>[2x]SNAMLDITTITRQNVTSVVGYYSDAKDDYYSKDSSFTSWQGTGAEALGLSGDVESARFKELLVGEIDTFTHMQRHVGDAKKERLGYDLTFSAPKGVSMQALIHGDKTIIEAHEKAVAAAVREAEKLAQARTTRQGKSVTQNTNNLVVATFRHETSRALDPDLHTHAFVMNM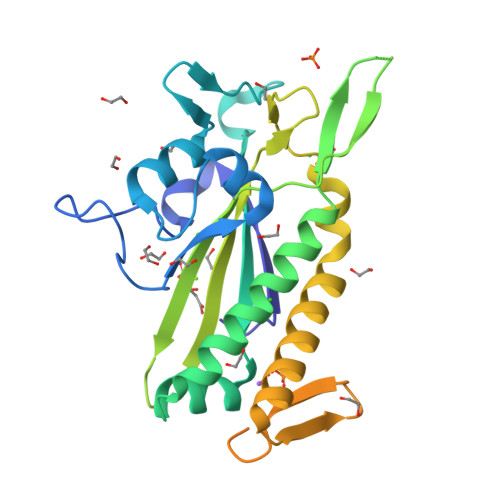TQREDGQWRALKNDELMRNKMHLGDVYKQELALELTKAGYELRYNSKNNTFDMAHFSDEQIRAFSRRSEQIEKGLAAMGLTRETADAQTKSRVSMATREKKTEHSREEIHQEWASRAKTLGIDFDNREWQG> GAQVSTQKTGAHESIIHYTNINYYKDAASNSANRQDFTQDPGK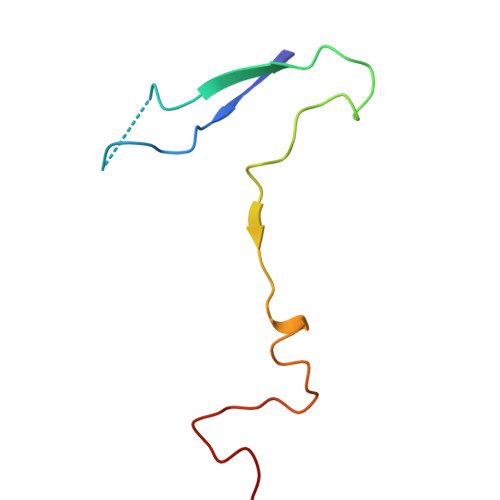FTEPVKDIMVKSLPALN> KTSDANETEDHLESLICKVGEKSACSLESNLEGLAGVLEADLPN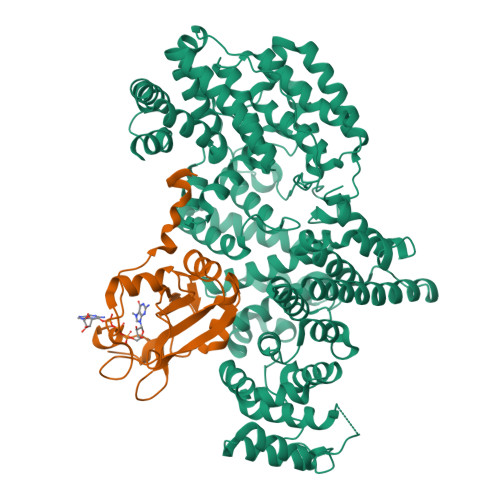YKSKILRLLCTVARLLPEKLTIYTTLVGLLNARNYNFGGEFVEAMIRQLKESLKANNYNEAVYLVRFLSDLVNCHVIAAPSMVAMFENFVSVTQEEDVPQVRRDWYVYAFLSSLPWVGKELYEKKDAEMDRIFANTESYLKRRQKTHVPMLQVWTADKPHPQEEYLDCLWAQIQKLKKDRWQERHILRPYLAFDSILCEALQHNLPPFTPPPHTEDSVYPMPRVIFRMFDYTDDPEGPVMPGSHSVERFVIEENLHCIIKSHWKERKTCAAQLVSYPGKNKIPLNYHIVEVIFAELFQLPAPPHIDVMYTTLLIELCKLQPGSLPQVLAQATEMLYMRLDTMNTTCVDRFINWFSHHLSNFQFRWSWEDWSDCLSQDPESPKPKFVREVLEKCMRLSYHQRILDIVPPTFSALCPSNPTCIYKYGDESSNSLPGHSVALCLAVAFKSKATNDEIFSILKDVPNPNQDDDDDEGFSFNPLKIEVFVQTLLHLAAKSFSHSFSALAKFHEVFKTLAESDEGKLHVLRVMFEVWRNHPQMIAVLVDKMIRTQIVDCAAVANWIFSSELSRDFTRLFVWEILHSTIRKMNKHVGAQSEQKNLFLVIFQRFIMILTEHLVRCETDGTSVLTPWYKNCIERLQQIFLQHHQIIQQYMVTLENLLFTAELDPHILAVFQQFCALQA;> MSGGLLKALRSDSYVELSQYRDQHFRGDNEEQEKLLKKSCTLYVGNLSFYTTEEQIYELFSKSGDIKKIIMGLDKMKKTACGFCFVEYYSRADAENAMRYINGTRLDDRIIRTDWDAGFKEGRQYGRGRSGGQVRDEYRQDYDAGRGGYGKLAQNQ>AISDADLKYLRRCVDLAREALDDGDEPFGSVLVDHTGTTLFE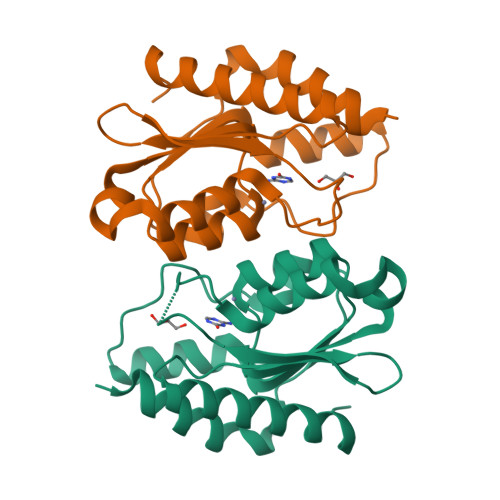DRNRVKDGDATAHPEFAIARWAARHLTPDRRARATVYTSGEHCPMCAAAHAWVGLGRIVYATSSAQLGGWLTEWGAQAPPVATLPINTVAPGVVVDGPAEELAETMHNLYRAKFGR[4x]>AYAQWVIIIIHNVGSKDVKIKNLKPSWGKLHADGDKDTEVSASKYEGTVIKPDEKLQINACGRSDAAEGTTGTFDLVDPADGDKQVRHFYWDCPWGSKTNTWTVSGSNTKWMIEYSGQNLDSGALGTITVDTLKK[26x];>QAGDTLNDVIQDPTRRNKLINDNNLLKGIIMGRDGPVPSSRELIVRPDTLRAIINNRATIETTTMEAEFTETLMESNYNSASVKVSAPFITANSEYSESSSFKNTETEKSMYTSSRYLFPQGRIDFTTPDSGFDDVIKLSPQFTSGVQAALAKATGTEKREALQNLFQEYGHVFRTKVHIGGVLSAHTMETFSRSENETEVKQDVKAGLEGAVKGWGGGATAGHGNTQGTITTSQNRKLNVKYIVNGGDYTKIQNTEEWVASTNQSEHWRVIEVTEVTAVADLLPQPIRGQVKDLLKPLLGKWVDVEKVPGLESLPVSVYRPKGAIPAGWFWLGDTADASKALLVKPTLPARSGRNPALTSLHQGSGMTEQPFVDLPQYQYLSTYFGSFA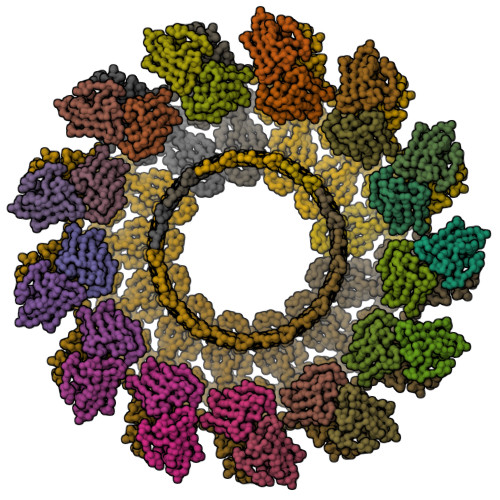HDTPPGSTLRGLRPDHVLPGRYEMHGDTISTAVYVTRPVDVPFPEDECFDLKSLVRVKLPGSGNPPKPRSALKKSMVLFDSGEK[12x];> SQAGDTLNDVIQDPTRRNKLINDNNLLKGIIMGRDGPVPSSRELIVRPDTLRAIINNRATIETTTMEAEFTETLMESNYNSASVKVSAPFITANSEYSESSSFKNTETEKSMYTSSRYLFPQGRIDFTTPDSGFDDVIKLSPQFTSGVQAALAKATGTEKREALQNLFQEYGHVFRTKVHIGGVLSAHTMETFSRSENETEVKQDVKAGLEGAVKGWGGGATAGHGNTQGTITTSQNRKLNVKYIVNGGDYTKIQNTEEWVASTNQSEHWRVIEVTEVTAVADLLPQPIRGQVKDLLKPLLGKWVDVEKVPGLESLPVSVYRPKGAIPAGWFWLGDTADASKALLVKPTLPARSGRNPALTSLHQGSGMTEQPFVDLPQYQYLSTYFGSFAHDTPPGSTLRGLRPDHVLPGRYEMHGDTISTAVYVTRPVDVPFPEDECFDLKSLVRVKLPGSGNPPKPRSALKKSMVLFDSGEK>[2x]MSEITLGKYLFERLKQVNVNTVFGLPGDFNLSLLDKIYEVEGMRWAGNANELNAAYAADGYARIKGMSCIITTFGVGELSALNGIAGSYAEHVG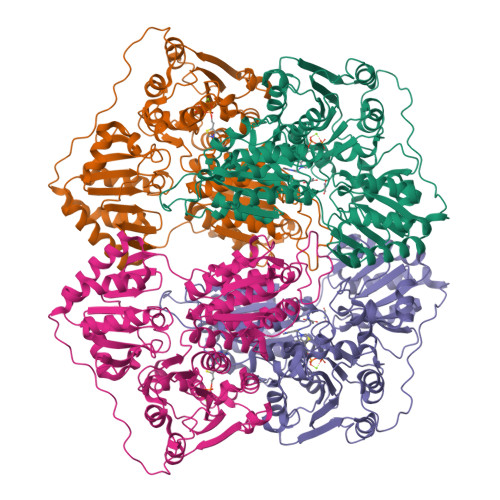VLHVVGVPSISAQAKQLLLHHTLGNGDFTVFHRMSANISETTAMITDIATAPAEIDRCIRTTYVTQRPVYLGLPANLVDLNVPAKLLQTPIDMSLKPNDAESEKEVIDTILVLIKDAKNPVILADACCSRHDVKAETKKLIDLTQFPAFVTPMGKGSIDEQHPRYGGVYVGTLSKPEVKEAVESADLILSVGALLSDFNTGSFSYSYKTKNIVEFHSDHMKIRNATFPGVQMKFVLQKLLTAIADAAKGYKPVAVPARTPANAAVPASTPLKQEWMWNQLGNFLQEGDVVIAETGTSAFGINQTTFPNNTYGISQVLWGSIGFTTGATLGAAFAAEEIDPKKRVILFIGDGSLQLTVQEISTMIRWGLKPYLFVLNNDGYTIEKLIHGPKAQYNEIQGWDHLSLLPTFGAKDYETHRVATTGEWDKLTQDKSFNDNSKIRMIEVMLPVFDAPQNLVEQAKLTAATNAKQ>[2x]MSGLHILAFGAHADDVEIGMAGTIAKYTKQGYEVGICDLTEADLSSNGTIELRKEEAKVAARIMGVKTRLNLAMPDRGLYMKEEYI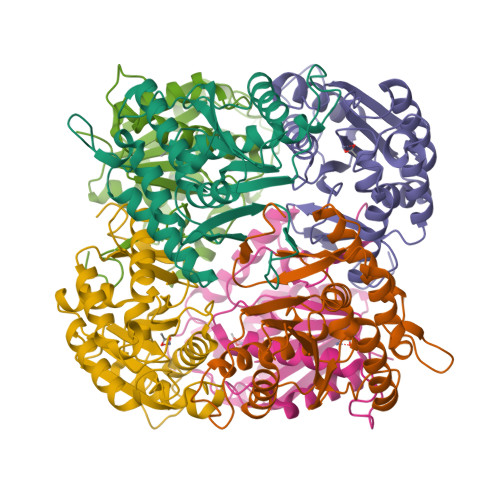REIVKVIRTYKPKLVFAPYYEDRHPDHANCAKLVEEAIFSAGIRKYMPELSPHRVESFYNYMINGFHKPNFCIDISEYLSIKVEALEAYESQFSTGSDGVKTPLTEGYVETVIAREKMFGKEVGVLYAEGFMSKKPVLLHADLLGGCKLGHHHHHH1-[(2S)-2,3-dihydro-1,4-benzodioxin-2-ylmethyl]-3-hydroxythieno[3,2-d]pyrimidine-2,4(1H,3H)-dione | C15 H12 N2 O5 S | 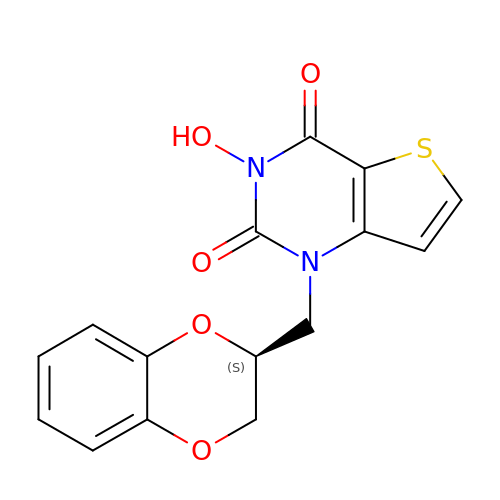MXQGCMQXTPTJJT-VIFPVBQESA-N2-naphthalen-2-yloxyethanoic 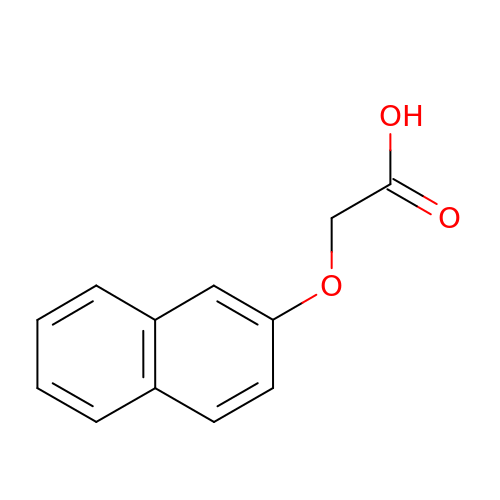acid | C12 H10 O3 | RZCJYMOBWVJQGV-UHFFFAOYSA-N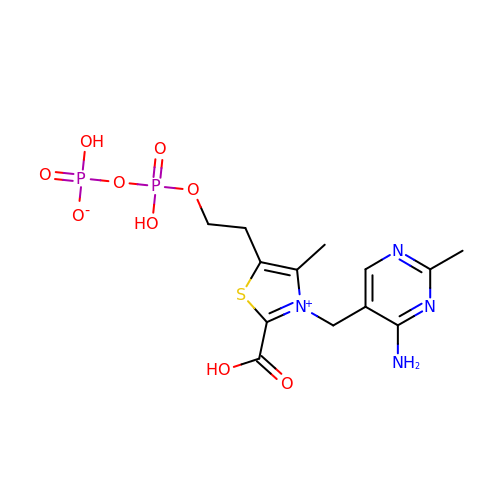[2-[3-[(4-azanyl-2-methyl-pyrimidin-5-yl)methyl]-2-carboxy-4-methyl-1,3-thiazol-3-ium-5-yl]ethoxy-oxidanyl-phosphoryl] hydrogen phosphate | C13 H18 N4 O9 P2 S | SXXTZHDPRYKKAS-UHFFFAOYSA-N>GQSAKEAIEAANADFVKAYNSKDAAGVASKYMDDAAAFPPDMARVDGRQNIQKLWQGAMDMGISELKLTTLDVQESGDFAFESGSFSLKAPGKDSKLVDAAGKYVVVWRKGQDGGWKLYRDIWNSDPAK[4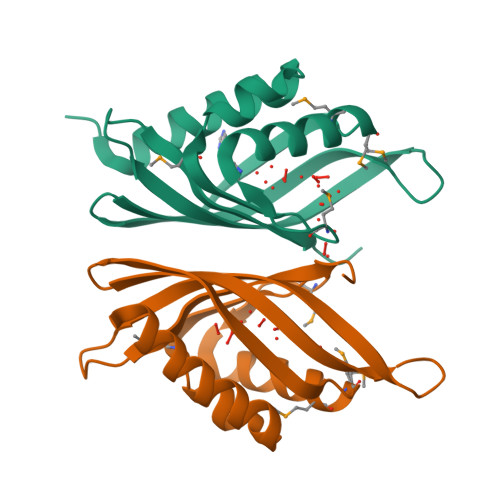x]>AECSVDIQGNDQMQFNTNAITVDKSCKQFTVNLSHPGNLPKNVMGHNWVLSTAADMQGVVTDGMASGLDKDYLKPDDSRVIAHTKLIGSGEKDSVTFDVSKLKEGEQYMFFCSELCGINHALMKGTLT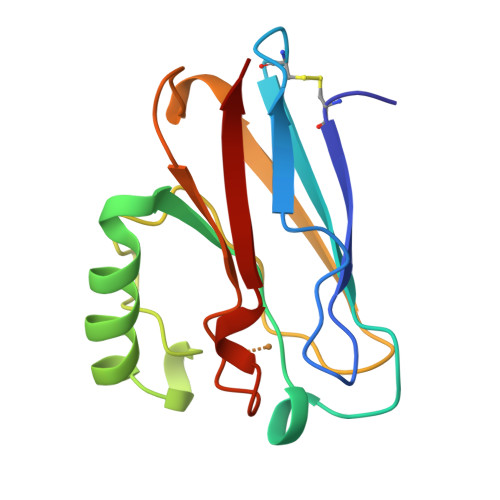LK[2x]Human endonuclease VIII-like 1 (hNEIL1) is a bifunctional DNA glycosylase of the Fpg/Nei family, which catalyzes the removal of damaged bases and subsequent incision of the newly generated abasic sites. Unlike traditional enzymes which are commonly referred to as highly specific biocatalysts, one special feature for hNEIL1 is its unique capability to recognize a wide range of substrates, including formamidopyrimidines, hydantoin lesions, oxidized, and dihydro-modified pyrimidine bases, derived from all four canonical bases. Here, by integrating structural, computational, and biochemical investigations, we show that hNEIL1 uses a triage mechanism to achieve broad specificity and reduce futile repair of normal bases. This mechanism involves two mutually competing interaction states: an activated state that commits catalysis and BER, and a quarantine state that temporarily separates and prevents the flipped base from catalysis via auto-inhibition.

To rule out the possibility that the observed interaction is caused by mutations introduced to hNEIL1 for crystallization experiments, we used an orthogonal approach in which a modified nucleobase substrate is bound by the native protein containing the wild type active site. We synthesized a 2′-fluoro-substituted stable mimic of DHU (FDHU), which allows binding but not catalysis by hNEIL1. Indeed, in the hNEIL1(R242)-FDHU structure, residues R242 and Y244 again swaps positions, recapitulating the observed 244-in conformation in the hNEIL1(R242)-DHU and hNEIL1(R242)-DHT structures. Apparently, the hydrogen bond interaction between residue 242 of hNEIL1 and the substrate which is present in the 242-in conformation is absent in the 244-in structures, indicating the loss of a key stabilizing factor of binding and catalysis. Thus, the 244-in conformation is incompetent of glycosylase activity and hence represents a distinct interaction mode with potentially special function. In contrast to the 242-in conformation, the 244-in conformation is catalytically inactive and functionally protects the nucleobase from cleavage, in competition with the activated state. In order to destabilize the quarantine state, we rationally designed hNEIL1(R242, G249P) and hNEIL1(R242, Y244H) to disrupt the flexibility of the loop or the aromatic stacking interactions respectively. Instead of the quarantine state originally observed in hNEIL1(R242)–FDHU structure, we found that both two mutants switched to the activated state as expected.

>MPEGPELHLASQFVNEACRALVFGGCVEKSSVSRNPEVPFESSAYRISASARGKELRLILSPLPGAQPQQEPLALVFRFGMSGSFQLVPREELPRHAHLRFYTAPPGPRLALCFVDIRRFGRWDLGGKWQPGRGPCVLQEYQQFRENVLRNLADKAFDRPICEALLDQRFFNGIGNYLRAEILYRLKIPPFEKARSVLEALQQHRPSPELTLSQKIRTKLQNPDLLELCHSVPKEVVQLGGRGYGSESGEEDFAAFRAWLRCYGMPGMSSLQDRHGRTIWFQGDPGPLAPKGRKS[3x]> GLAGLVPAPDHGMREEILGDRSRLIRQRGEHALIGISAGNSYFSQKNTVMLLQWAGQRFERTDVVYVDTHIDEMLIADGRSAQEAERSVKRTLKDLRRRLRRSLESVGDHAERFR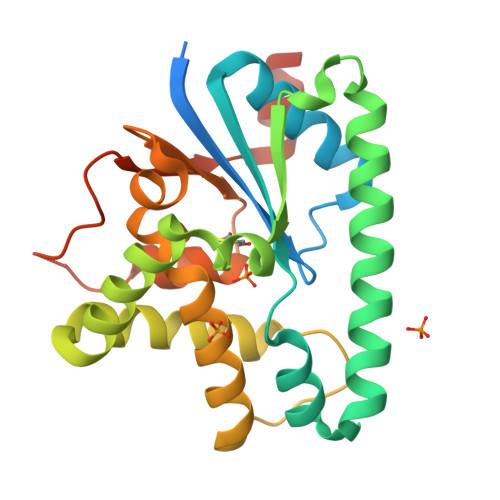VRSLSELQETPEYRAVRERTDRAFEEDAEFATACEDMVRAVVMNRPGDGVGISAEHLRAGLNYVLAEAPLFADSPGVFSVPSSVLCYHIDTPITAFLSRRETGFRAAEGQAYVVVRPQELADAARSHHHHHH> MSSERACMLCGIVQTTNEFNRDGCPNCQGIFEEAGVS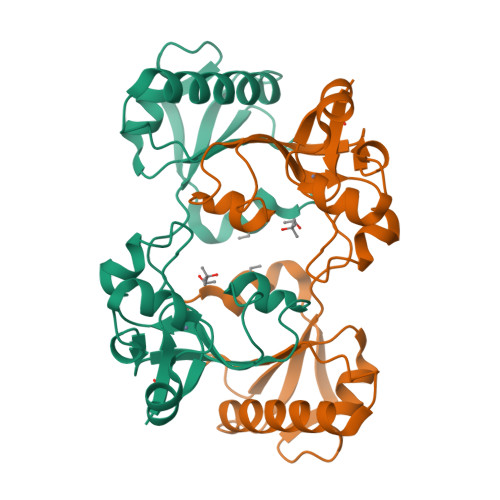TMECTSPSFEGLVGMCKPTKSWVAKWLSVDHSIAGMYAIKVDGRLPAEVVELLPHYKPRDGSGSATIWGVRCRPGKEKELIRKLLKKKFNLDRAMGKKKLKILSIFQRDNYTGRIYIEAPKQSVIEKFCNGVPDIYISQKLLIPVQELPLLLKPNLEHHHHHH> SNAMKPDIYENNREGILCVYKNEKWLVCIKNWKPDNDIEGIAHLEIHHSTDEQFILSAGKAILITAEKENDKFNIELTLMEKGKVYNVPAECWFYSITQKDTKMMYVQDSNCSM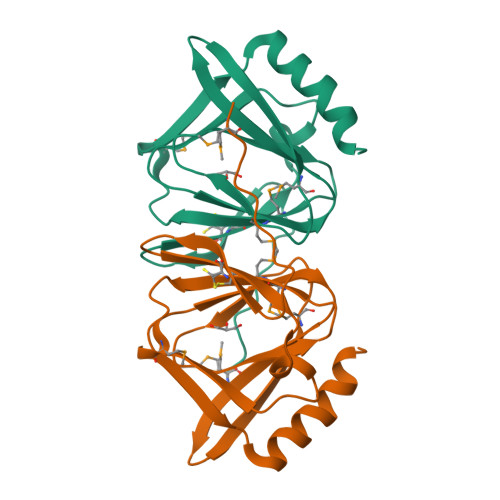DNSDFCDLSKEEIEYIQTNARKLFEK> IKTVLDTAQAPYKGSTVIGHALSKHAGRHPEIWGKVKGSMSGWNEQAMKHFKEIVRAPGEFRPTMNEKGITFLEK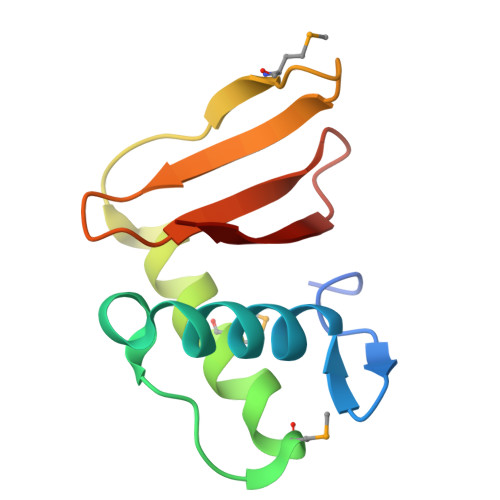RLIDGRGVRLNLDGTFKGFID> XVTIDADLMDAADLLEGEQVTIVDIDNGARLVTYAITGERGSGVIGINGAAAHLVHPGDL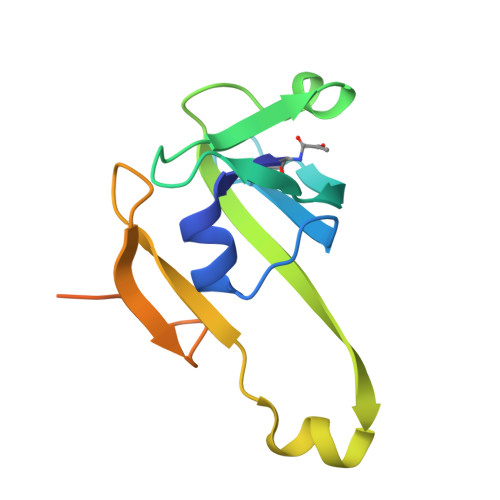VILIAYATMDDARARTYQPRIVFVDAYNKPIDIGHDPAFVPENAGELLDPRLGVGLEHHHHHH>GSHMASPNGQTKPLPALKLALEYIVPAMNKHGICVVDDFLGKETGQQIGDEVRALHDTGKFTDGQLVSQKSDSSKDIRGDKITWIEGK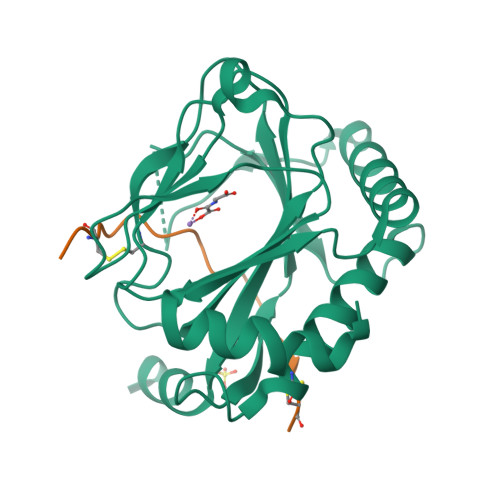EPGCETIGLLMSSMDDLICHCNGKLGSYKINGRTKAMVACYPGNGTGYVRHCDNPNGDGRCVTCIYYLNKDWDAKVSGGILRIFPEGKAQFADIEPKFDRLLFFWSDRRNPHEVQPAYATRYAITVWYFDADERAAAKVKYLTGEKGVRVELNKPSDSVGKDVF[2x];>DACTLLAPAAGDTIISLCF[2x]> MNVVDISRWQFGITTVYHFIFVPLTIGLAPLIAVMQTLWVVTDNPAWYRLTKFFGKLFLINFAIGVATGIVQEFQFGMNWSEYSRFVGDVFGAPLAMEGLAAFFFESTFIGLWIFGWNRLPRLVHLACIWIVAIAVNVSAFFIIAANSFMQHPVGAHYNPTTGRAELSSIVVLLTNNTAQAAFTHTVSGALLTAGTFVAAVSAWWLVRSSTTHADSDTQAMYRPATILGCWVALAATAGLLFTGDHQGKLMFQQQPMKMASAESLCD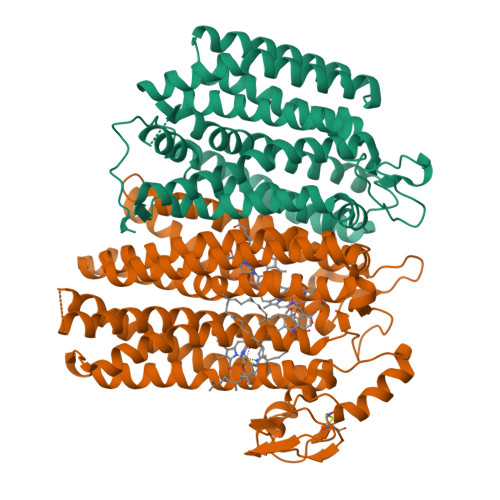TQTDPNFSVLTVGRQNNCDSLTRVIEVPYVLPFLAEGRISGVTLQGIRDLQQEYQQRFGPNDYRPNLFVTYWSFRMMIGLMAIPVLFALIALWLTRGGQIPNQRWFSWLALLTMPAPFLANSAGWVFTEMGRQPWVVVPNPTGDQLVRLTVKAGVSDHSATVVATSLLMFTLVYAVLAVIWCWLLKRYIVEGPLEHDAEPAAHGAPRDDEVAPLSFAY;> MVLQELWFGVIAALFLGFFILEGFDFGVGMLMAPFAHVGMGDPETHRRTALNTIGPVWDGNEVWLITAGAAIFAAFPGWYATVFSALYLPLLAILFGMILRAVAIEWRGKIDDPKWRTGADFGIAAGSWLPALLWGVAFAILVRGLPVDANGHVALSIPDVLNAYTLLGGLATAGLFSLYGAVFIALKTSGPIRDDAYRFAVWLSLPVAGLVAGFGLWTQLAYGKDWTWLVLAVAGCAQAAATVLVWRRVSDGWAFMCTLIVVAAVVVLLFGALYPNLVPSTLNPQWSLTIHNASSTPYTLKIMTWVTAFFAPLTVAYQTWTYWVFRQRISAERIPPPTGLARRAP Here, we report that the outer membrane lipoprotein QseG functions as an accessory protein that directly binds to and activates the histidine kinase QseE via its C-terminal domain. QseEF, a TCS responsive to multiple ligands including phosphate, sulfate, adrenaline, and AI-3, is essential for the virulence of pathogenic Enterobacteriaceae. Notably, genomic analyses reveal that a third gene qseG is co-transcribed with qseE and qseF, encoding an outer membrane lipoprotein anchored to the inner leaflet via N-terminal lipid modification. Collectively, our findings establish QseG as an endogenous activator of the QseEF signaling pathway via a conserved regulatory mechanism.

To refine atomic modeling, we additionally determined the crystal structures of QseG37-221 at 2.1 Å and the QseE sensor domain at 2.4 Å resolution. The lipoprotein QseG is anchored in the outer membrane, facing the periplasm under physiological conditions, with residues 1-36 comprising its signal sequence. The N-terminal region of each monomer QseG forms a globular fold with α-helices, whereas the C-terminus adopts a two-helix bundle, with each monomer contributing a long parallel helix. Following cleavage of the secretion signal peptide, the first N-terminal cysteine (herein, Cys37 within the long N-terminal loopC37-E57 of QseG in S. Typhimurium SL1344) undergoes lipidation, thereby anchoring QseG to the inner leaflet of the bacterial outer membrane. QseG37-end and QseG37-221 retained QseE-binding capability, whereas further C-terminal truncations (QseG37-214, QseG37-193, and QseG37-181) abolished this interaction. Consistent with the pull-down results, only QseG truncations that retained QseE-binding capacity induced autophosphorylation. These findings indicate that the QseG C-terminus is essential for QseE activation, highlighting QseG’s critical role in the QseEF TCS regulatory pathway. To assess the functional significance of the QseG-QseE interface, we introduced site-directed mutations in key QseG residues (L209D, E213A, R214A, R219A, and K220A) predicted to be essential for complex formation. Notably, the L209D and R219A mutations completely disrupted QseG-QseE complex formation (lanes 2, 9, 10, 13) and significantly reduced QseE autophosphorylation (lanes 2–4, lanes 1–3, 6). These findings highlight the crucial role of Leu209 and Arg219 in stabilizing the QseG-QseE interaction and activating QseE’s autokinase function.

>[2x]CVPHASQQLPGSAAQDTLPHYQLADYLPTACADIWSLRGQAVETNPLYWLRTIDCADRLMPVQSRAEARALTDDNWQNAFRRGILLADAKITPPERRAIVTRLEALSAQIPAQVRPVYQIWHDGQALQLALSAERQRYSKLQQMSDSELDALRQQQQALQTQLDLTTRKLESLTDIERQLSTRKPLE>[2x]MAEKALATLKELA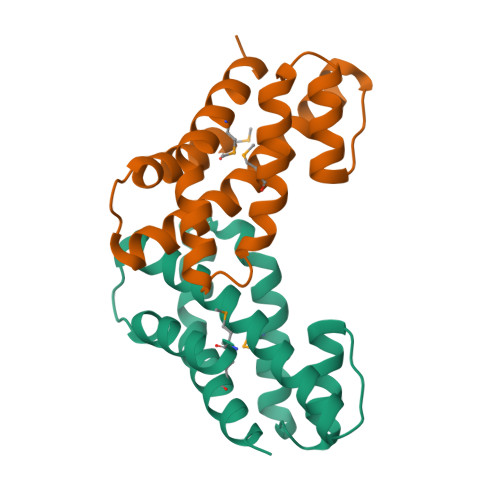FLEDPSPVERDAAIQRFEYTFEAFWKALQAYLREKEGLEGASPKGVIRLAREVGLLRDEEARLALGMVDDRSLTVHTYNEPLARAIFRRLPDYARLMEQVLGRLRR> PEIGNNGAEKQISLHKGQPFIDTQDVGAADPNTPAVTIEGPSDYVIAIDAGTPVAPEFRDANGDKLDPSTRVTIQKCDKQGN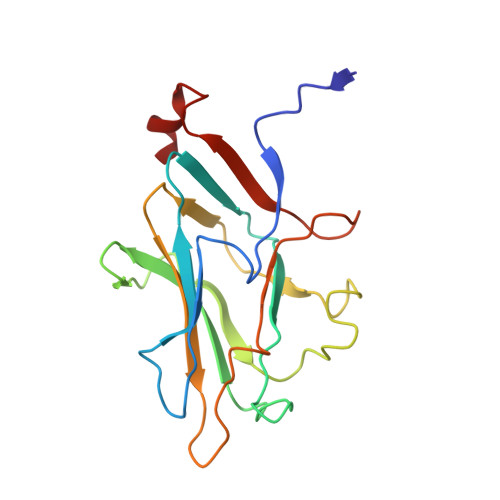PLGDGIVFSDTLGRFEYSKMRSDPDYMRKTTTSLMIDEREIVKIFVEVPPNANGMDADNSRITIGDDTSDYGKAVGIVEHGDLSPAESKA> AISIKTPEDIEKMRVAGRLAAEVLEMIEPYVKPGVSTGELDRICNDYIVNEQHAVSACLGYHGYPKSVCISINEVVCHGIPDDAKLLKDGDIVNIDVTVIKDGFHGDTSKMFIVGKPTIMGERLCRITQESLYLALRMVKPGINLREIGAAIQKFVEAEGFSVVREYCGHGIGRGFHEEPQVLHYDSRETNVVLKPGMTFTIEPMVNAGKKEIRTMKDGWTVKTKDRSLSAQYEHTIVVTDNGCEILTLRKDDTIPAIISHD

Methionine aminopeptidase (MetAP) removes the N-terminal methionine residue from nascent proteins in all types of cells. MetAP is therefore a potential target for developing novel broad spectrum antibacterial drugs. E. coli MetAP is a typical bacterial MetAP, containing only a catalytic domain. A surface-exposed loop containing Y62, H63, G64 and Y65 (the YHGY loop) is an integral part of the active site pocket.

We report here five new X-ray crystal structures of the Mn(II)-form of E. coli MetAP, each complexed with a different inhibitor. All eight structures, including the five new ones, have the typical "pita-bread" fold found in other MetAP structures, and each of them contains two Mn(II) ions at the dinuclear metal site. A single molecule of inhibitor sits in the shallow active site pocket. Common features of the Mn(II)-form selective inhibitors 4–8 bound to E. coli MetAP in the five new structures are that all use their carboxylate group to coordinate with the two Mn(II) ions at the dinuclear metal site and all take a non-coplanar or twisted conformation for the two aromatic rings, consistent with our previously reported structures of E. coli MetAP complexed with 1–3. The twisted conformation found in all of the Mn(II)-form-selective inhibitors 1–8 is in agreement with the requirement of a hydrophobic ortho-substitution, such as chlorine, on the phenyl ring for inhibitory activity. The twist angles observed in the MetAP complexes of 1–8 range from the smallest 23.3° for 6 to the largest 52.9° for 4, suggesting that in general, the phenylfuran-based inhibitors dock into the active site in a conformation that may correspond to a minimum-energy solution conformation. The residues forming the dinuclear metal site (H171, D108, E204, E235 and D97), as well as the nearby residues S110, T202, F177, H178 and H79, show little change in position upon binding of any of these inhibitors. In contrast, residues Y62, H63, G64, and Y65 in the YHGY loop, as well as residue W221, moved significantly. The same is true for other inhibitors, and the loop show a great adaptability. This flexibility allows the binding pocket to adapt to different shapes of the bound inhibitors.> MKYLLPTAAAGLLLLAAQPAMAMDGGPDTVAPPKQAQAIDSTHECHLCGMLITEFPGPKGELYTK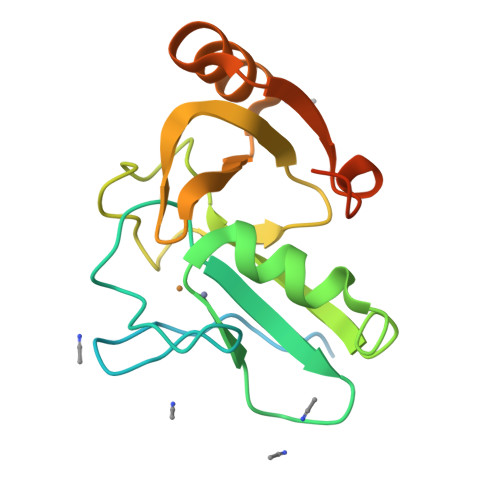TSEKVKNFCSTRDLFSFLLDPEYVHQVKEVYVHDMSLSPWAKPNDSHFINARLAWFVVGSSQTGAMGETIGSFSVKKDAEAFIEQYGGKLYRFDEITQAQLLENLYFQSWSHPQFEK5-benzyl-2-(3-fluoro-2-hydroxyphenyl)-6-methyl-3-(2-phenylethyl)pyrimidin-4(3H)-one | C26 H23 F N2 O2 | 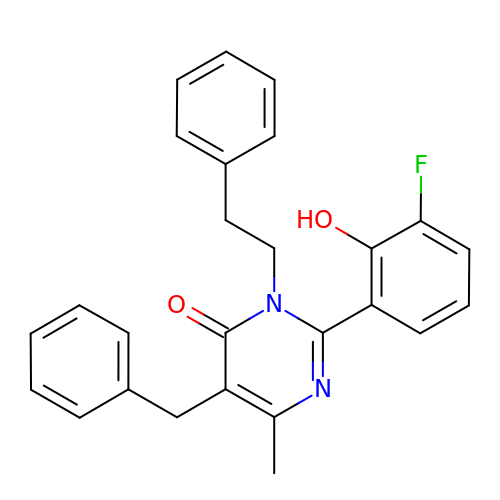BFDADFMMNADXMI-UHFFFAOYSA-N> MADDEVVDPKKYLEESCKPKCVKPLLEY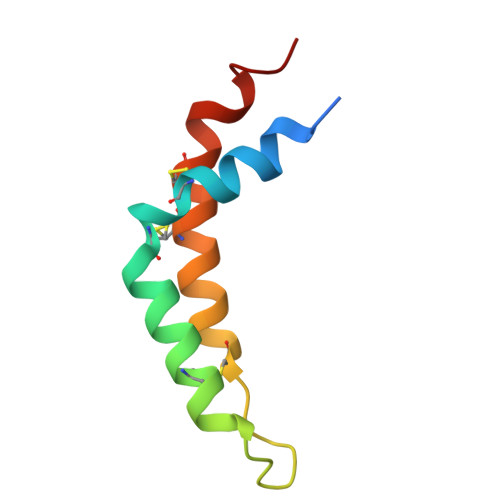QACVKRIQGDDSGHKHCTGQYFDYWQCIDKCVAPKLFAKLK>DRVYIHPFHLLYHNKSTCAQLENPSVETLPESTFEPVPIQAKTSPVNEKTLHDQLVLAAEKLEDEDRKRAAQVAMITNFVGFRMYKMLNEAGSGASGAILSPPALFGTLVSFYLGSLDPTASQLQTLLDVPVKEGDCTSRLDGHKVLAALRAVQGLLVTQGGSSSQTPLLQSIVVGLFTAPGFRLKHSFVQSLALFTPALFPRSLDLSTDPVLATEKINRFIKAVTGWKMNLPLEGVSTDSTLLFNTYVHFQGTMRGFSQL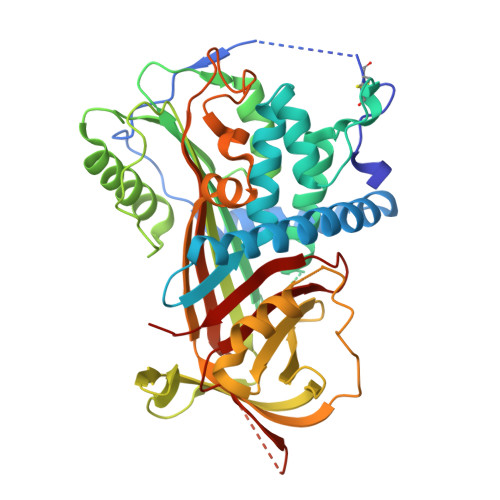PGVHEFWVDNSISVSVPMISGTGNFQHWSDAQNNFSVTCVPLGERATLLLIQPHCISDLDRVEALIFQNDLLTWIENPPPRAIRLTLPQLEIRGSYNLQDLLAEDKLPTLLGAEANLNNIGDTNPRVGEVLNSILLELKAGEEEQPTTSVQQPGSPEALDVTLSSPFLFAIYEQDSGTLHFLGRVNNPQSVV[4x]>[4x]ADFEVHMLNKGKDGAGVFEPASLKVAPGDTVTFIPTDKGHN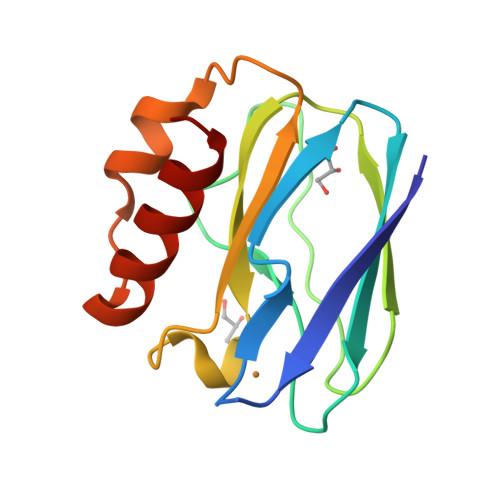VETIKGMIPDGAEAFKSKINENYKVTFTAPGVYGVKCTPHYGMGMVGVVQVGDAPANLEAVKGAKNPKKAQERLDAALAALGN>[6x]MGSDKIHHHHHHMAFFDLPLEELKKYRPERYEEKDFDEFWEETLAESEKFPLDPVFERMESHLKTVEAYDVTFSGYRGQRIKGWLLVPKLEEEKLPCVVQYIGYNGGRGFPHDWLFWPSMGYICFVMDTRGQGSGWLKGDTPDYPEGPVDPQYPGFMTRGILDPRTYYYRRVFTDAVRAVEAAASFPQVDQERIVIAGGSQGGGIALAVSALSKKAKALLCDVPFLCHFRRAVQLVDTHPYAEITNFLKT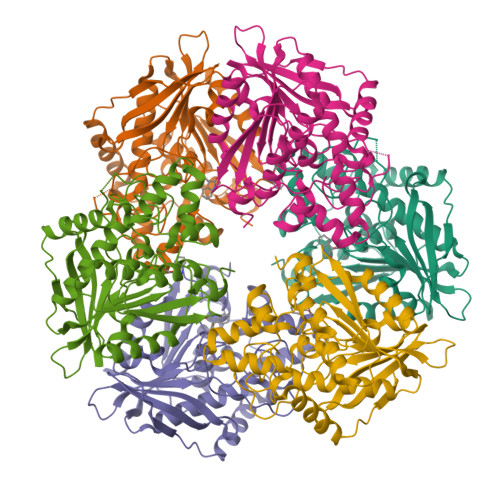HRDKEEIVFRTLSYFDGVNFAARAKIPALFSVGLMDNICPPSTVFAAYNYYAGPKEIRIYPYNNHEGGGSFQAVEQVKFLKKLFEKG> GRC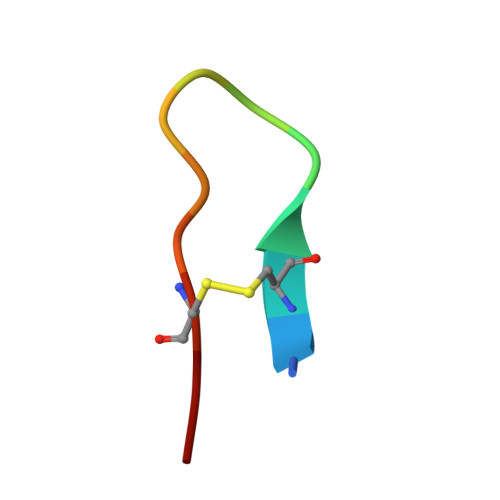TKSIPPICFP>GPLGSPEFGYWITCCPTCDVDINTWVPFYSTELNKPAMIYCSHGDGHWVHAQCMDLEERTLIHLSEGS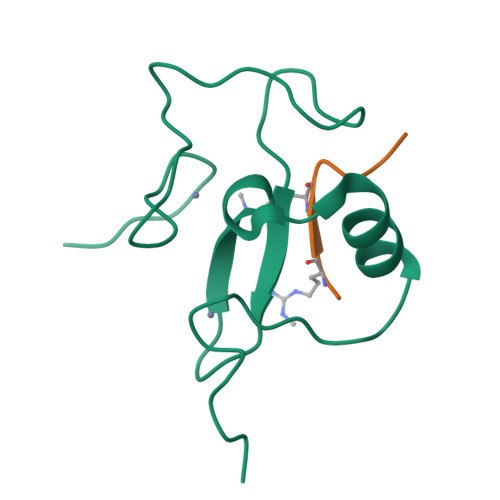NKYYCNEHVQIARA[2x];>[2x]ARTKQTAA> GPGSMPPPSDIVKVAIEWPGA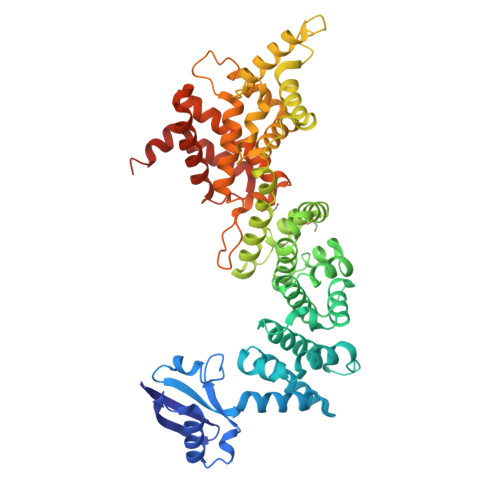NAQLLEIDQKRPLASIIKEVCDGWSLPNPEYYTLRYADGPQLYITEQTRSDIKNGTILQLAISPSRAARQLMERTQSSNMETRLDAMKELAKLSADVTFATEFINMDGIIVLTRLVESGTKLLSHYSEMLAFTLTAFLELMDHGIVSWDMVSITFIKQIAGYVSQPMVDVSILQRSLAILESMVLNSQSLYQKIAEEITVGQLISHLQVSNQEIQTYAIALINALFLKAPEDKRQDMANAFAQKHLRSIILNHVIRGNRPIKTEMAHQLYVLQVLTFNLLEERMMTKMDPNDQAQRDIIFELRRIAFDAESDPSNAPGSGTEKRKAMYTKDYKMLGFTNHINPAMDFTQTPPGMLALDNMLYLAKVHQDTYIRIVLENSSREDKHECPFGRSAIELTKMLCEILQVGELPNEGRNDYHPMFFTHDRAFEELFGICIQLLNKTWKEMRATAEDFNKVMQVVREQITRALPSKPNSLDQFKSKLRSLSYSEILRLRQSERMSQDD> MTKNPRNNKPKKILDSSYKSKTIWQNYIDALFETFPQLEISEVWAKWDGGNVTKDGGDAKLTANIRTGEHFLKAREAHIVDPNSDIYNTILYPKTGADLPCFGMDLMKFSDKKVIIVFDFQHPREKYLFSVDGLPEDDGKYRFFEMGNHFSKNIFVRYCKPDEVDQYLDTFKLYLTKYKEMIDNNKPVGEDTTVYSDFDTYMTELDPVRGYMKNKFGEG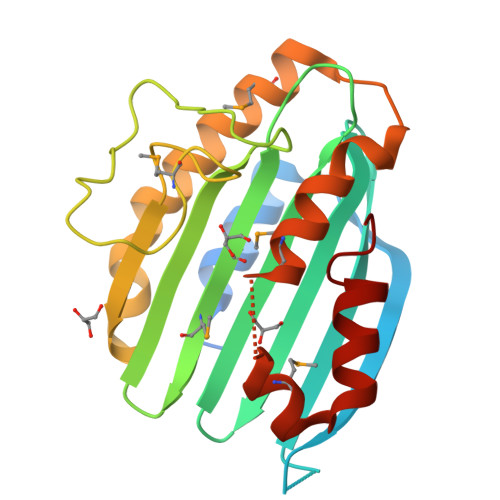RSEAFVNDFLFSYK> GGIQDSSCT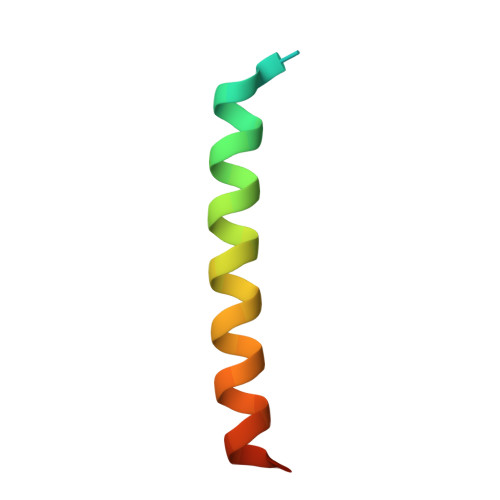RDDRRERIVAECNAVRQALQDLLSEYMGNAG METHYL 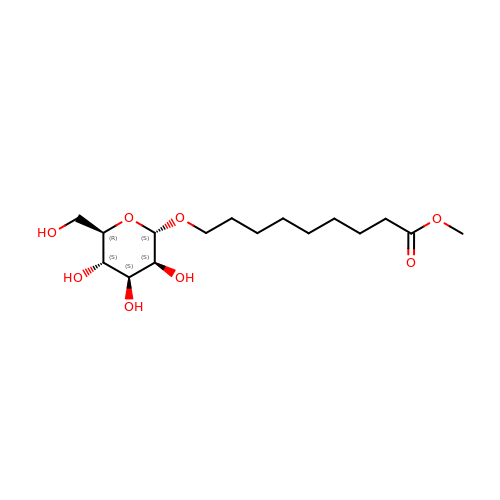ESTER OCTYL ALPHA-1O-D-MANNOPYRANNOSIDE | C16 H30 O8 | ZJZBQHWSENWEMY-VMMWWAARSA-N> GMGSMSTPAASANGGQVLLLPFPAAQGHTNPMLQFGRRLAYHGLRPTLVTTRYVLSTTPPPGDPFRVAAISDGFDDASGMAALPDPGEYLRTLEAHGARTLAELLL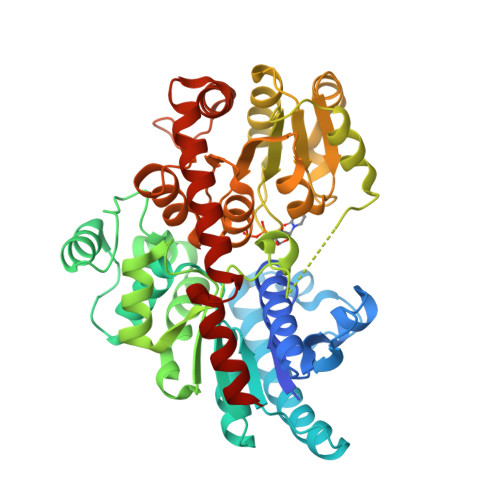SEARAGRPARVLVYDPHLPWARRVARAAGVATAAFLSQPCAVDLIYGEVCARRLALPVTPTDARGLYARGVLGVELGPDDVPPFVAAPELTPAFCEQSIEQFAGLEDDDDVLVNSFSDLEPKEAAYMESTWRAKTIGPSLPSFYLDDGRLRSNTAYGFNLFRSTVPCMEWLDKQPPRSVVLVSYGVVSTFDVAKLEELGNGLCNSGKPFLWVVRSNEEHKLSVQLRKKCEKRGLIVPFCPQLEVLAHKATGCFLSHCGWNSTLEAIVNGVPLVAMPHWADQPTISKYVESLWGMGVRVQLDKSGILQREEVERCIREVMDGDRKEDYRRNATRLMKKAKESMQEGGSSDKNIAEFAAKYSN> MADYKDDDDKSGP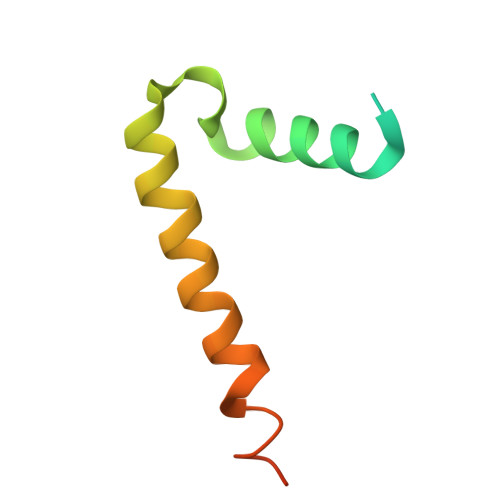DEVDASGRMNWVQRKIYLYNVTFGLYMLDWWERYLFNSLVVVLMWFVLYNGTRYFSELFQRHLT> GSMADEATRRVVSEIPVLKTNAGPRDRELWVQRLKEEYQSLIRYVENNKNADNDWFRLESNKEGTRWFGKCWYIHDLLKYEFDIEFDIPITYPTTAPEIAVPELDGKCAKMYRGGKIC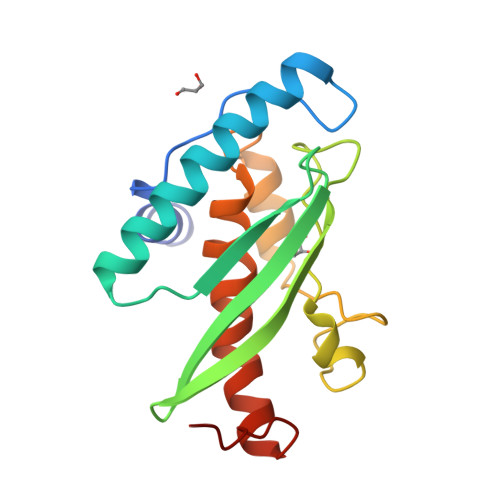LTDHFKPLWARNVPKFGLAHLMALGLGPWLAVEIPDLIQKGVIHHKEKCNQ> GDIVMKEKPKVTLNEIVGLEDVKEALKEAVVYPSKRPDLFPLGWPRGILLYGPPGCGKTMIAAAVANELDSEFIHVDAASIMSKWLGEAEKNVAKIFKTARELSKKENKPAIIFIDELDALLASYTSEVGGEARVRNQFLKEMDGLADKNEISKVYVIGATNKPWRLDEPFLRRFQKRIYITLPDKAHRL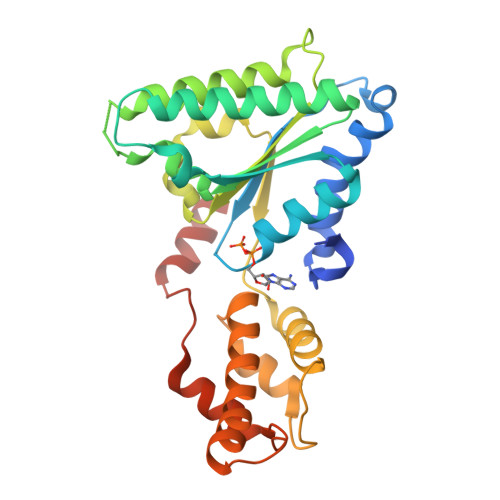ELLKHYSSKVKLDPNVNLEELAELTDGYTASDIRDIVQSAHMRVVKEMFEKNLQEPRAINMDDFREVLKVRKPSVNQDMLKAYAAWHEKFKAL>MIHLTSVEASVSFENGKIVVRLPITRPTSKIRVKKIENGVGIPVSTRKKSFPSDENLRDYYIEWQISYARDGKYDYELSRMVRLAHEHGILTYNDIYELLKFADDVKSYLEDKGIRRESTNEELYGFNIYEDVYPVAKKELPSGEFIGIVLK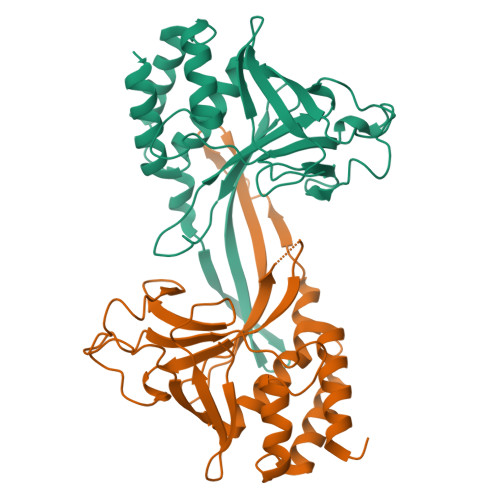HKQRAVGYQSMVYVCIPLTNVEPSLAGRVARRNEVVKYEVPVDLMKELLKAFIIASETHKNDIVKFLRSIIGTS[6x]> DYKDDDDAMGRSHTITMTTTSVSSWPYSSHRMRFITNHSDQPPQNFSATPNVTTCPMDEKLLSTVLTTSYSVIFIVGLVGNIIALYVFLGIHRKRNSIQIYLLNVAIADLLLIFCLPFRIMYHINQNKWTLGVILCKVVGTLFYMNMYISIILLGFISLDRYIKINRSIQQRKAITTKQSIYVCCIVWMLALGGFLTMIILTLKKGGHNSTMCFHYRDKHNAKGEAIF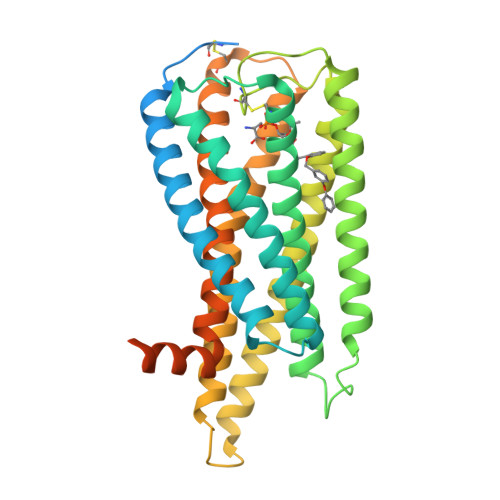NFILVVMFWLIFLLIILSYIKIGKNLLRISKRRSKFPNSGKYATTARNSFIVLIIFTICFVPYHAFRFIYISSQLNVSSCYWKEIVHKTNEIMLVLSSFNSCLDPVMYFLMSSNIRKIMCQLLFRRFQGEPSRSESTSEFKPGYSLHDTSVAVKIQSSSKSTENLYFQ> GUUGCAGUGAGAGAAAGAAGUACUUGCGUUACCUCAUGAAAGCGACCUUAGGGCGGUGUAAGCUAAGGAUGAGCACGCAACGAAAGGCAUUCUUGAGCAAUUUUAAAAAAGAGGCUGG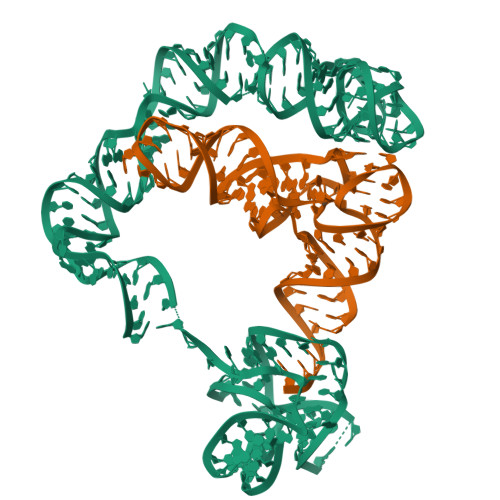GAUUUUGUUCUCAGCAACUAGGGUGGAACCGCGGGAGAACUCUCGUCCCUA;> GCGGAAGUAGUUCAGUGGUAGAACACCACCUUGCCAAGGUGGGGGUCGCGGGUUCGAAUCCCGUCUUCCGCUCCA> MAHHHHHHMDPQSTAAATVLKRAVELDSESRYPQALVCYQEGIDLLL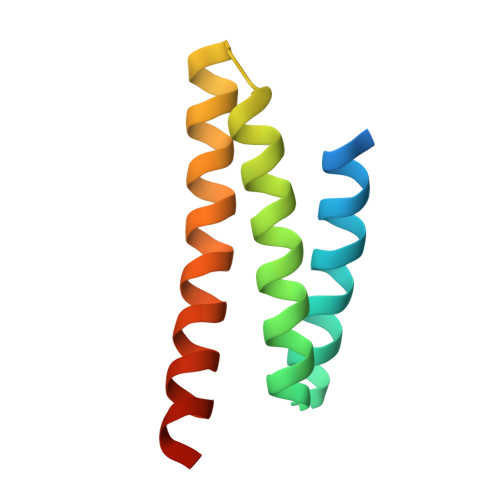QVLKGTKDNTKRCNLREKISKYMDRAENIKKYLDQEKED> RKTGLKQKIVIKVAMEGNNCRS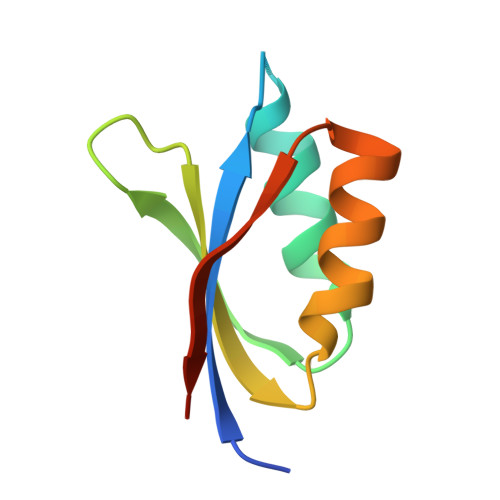KAMALVASTGGVDSVALVGDLRDKIEVVGYGIDPIKLISALRKKVGDAELLQVSQAKED>[2x]SAFPIDLRGQTAFVAGVADSHGYGWAIAKHLASAGARVALGTWPPV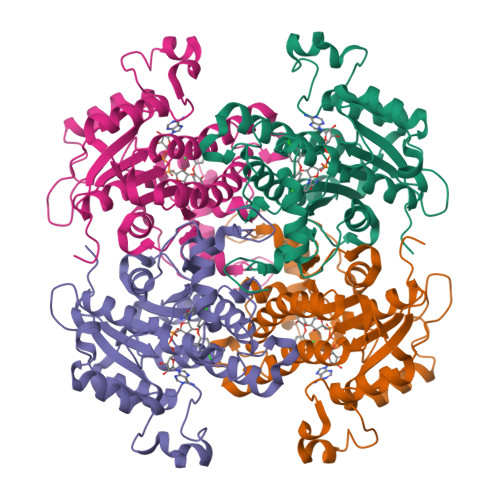LGLFQKSLQSGRLDEDRKLPDGSLIEFAGVYPLDAAFDKPEDVPQDIKDNKRYAGVDGYTIKEVAVKVKQDLGNIDILVHSLANGPEVTKPLLETSRKGYLAASSNSAYSFVSLLQHFGPIMNEGGSAVTLSYLAAERVVPGYGGGMSSAKAALESDTRTLAWEAGQKYGVRVNAISAGPLKSRAASAIGKSGEKSFIDYAIDYSYNNAPLRRDLHSDDVGGAALFLLSPLARAVSGVTLYVDNGLHAMGQAVDSRSMPPLQRATQEIN>[2x]GSDSSVNVALQASFDAGPYLLELLEAAAAENASSYFPLLDRIAEGVLDDAVTEKELYDRFLTIVQDEGHINDAADLSSFKFSLAIRSAVPRVEAHYQYYNTSVEPRLGTAQDAACPVWVHMDGMQYCSPTLERAQQAVSADLEARDLPFDRKLGDPTAPLAILYADVASPAFGEYHRKLSAMAKEGQVSYVVRYRPPPSASFRPLFLAGYGVELTLKRTDYIMIDDREAEESNEKQTNKRKVGSPSADELEEESPPDLKPLSSSEVARLGMNAASFILDSPDPFATLTKLSQDFPKYSSAVAAYNVTQEFLDEYYANRAASLPGGRNVLWINGLQIDSRQVDAYSLLEHLRHERQFIGQFRKLGLSNIEALDLLLHPNLTDGQSDAETQRYDWRDEVEGGDVIIWLNDLTKDKRYSDFPSDIDALLQPTYPGQLPAVRRDVHNVVIPIDLTNEDDVYMVVQHIQTFIKRLIPVRFGLVPLVHSEPAKSQAKIARYLQMTHGLAAMMKYFQRALEKDKLARPDQ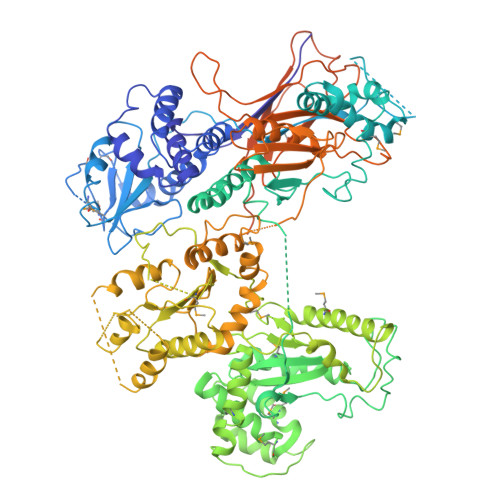ALFDETIASARVLRGKAQSFEEALSSTTLEEVMDKTGRYIKRLDLGGRSPPVLANGVLLGRGDNFLQELSMRVAIDLQLIQQSIVQDAVEEDTWLPSYFLSQAALTRNELIMPQDPSKIRIVNLVQVAESHDLTSLLRISAEGPGTNSLLMAVVGDFDSEAGLNLLISALKFRLAHPEIEVVPLHTSDDETNTHVSSQLYQLLRTERVDASEILEKIQIIKSTSDIGATATSKELAYWAQTKQLAADLGYPSGTRGVLLNGRAVGPVPSTSTLAEDDLEILLAYEFSKRLGTVAKVMKDLNLGHKVAGSVEFAKLTSLVALSTTSDIPEGIFESRSKYRQSAIKTWNGAHSAITVSHSDDASINIVATIDPASERSQRWVPILRTLSKLNGVNVKIFLTPVRILQELPIKRFYRHVLEPEPSFDEHGALNRPGASFSRLPEDALLTLGMDVPPSWLVSPKESVHDLDNIRLSSLREGSDVDAIYELEHILIEGHSTDVTTRSAPRGVQLLLGTDKNPHFADTIVMANLGYFQFKARPGFWKINLKPGPSQRIFNLDSVGGMGYQPKPGDETNEVALTSFQGRTLFPRLSRKPGHEEDDVLETGPKPG>[2x]ATFDILNKCTYTVWAAASPGGGRRLDSG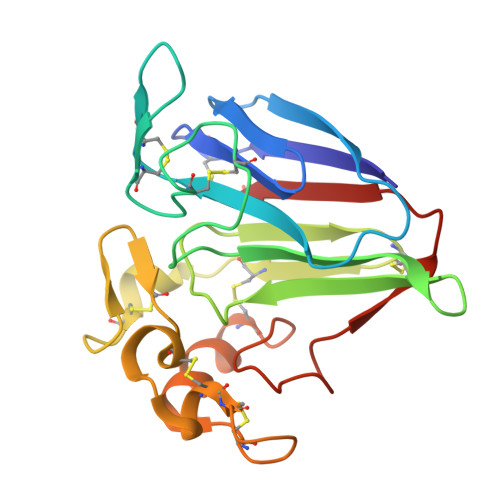QSWTITVNPGTTNARIWGRTSCTFDANGRGKCETGDCNGLLECQGYGSPPNTLAEFALNQPNNLDYIDISLVDGFNIPMDFSGCRGIQCSVDINGQCPSELKAPGGCNNPCTVFKTNEYCCTDGPGSCGPTTYSKFFKDRCPDAYSYPQDDKTSLFTCPSGTNYKVTFCP> ADKELKFLVVD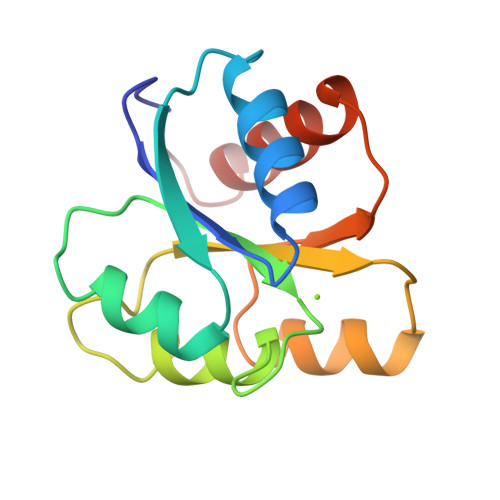DFSTMRRIVRNLLKELGFNNVEEAEDGVDALNKLQAGGFGFIISDWNMPNMDGLELLKTIRADSAMSALPVLMVTAEAKKENIIAAAQAGASGYVVKPFTAATLEEKLNKIFEKLGM> GGSGSMALIMEPVSKWSPSQVVDWMKGLDDCLQQYIKNFEREKISGDQLLRITHQELEDLGVSRIGHQELILEAVDLLCALNYGLETENLKTLSHKLNASAKNLQNFITGRRRSGHYDGRTSRKLPNDFLTSVVDLIGAAKSLLAWLDRSPFAAVTDYSVTRNNVIQLCLELTTIVQQDCTVYETENKILHVCKTLSGVCDHIISLSSDPLVSQSAHLEVIQLANIKPSEGLGMYIKSTYDGLHVIT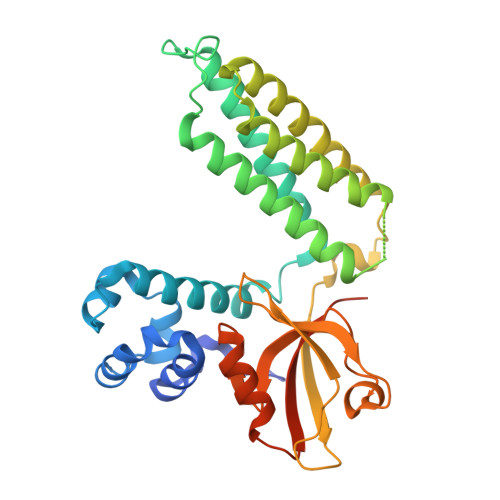GTTENSPADRCKKIHAGDEVIQVNHQTVVGWQLKNLVNALREDPSGVILTLKKRPQSMLTSAPALLKNMRWK>[2x]MKMNVESF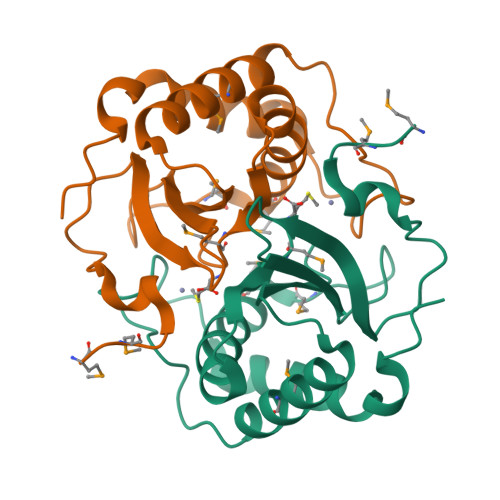NLDHTKVKAPYVRIADRKKGVNGDLIVKYDVRFKQPNRDHMDMPSLHSLEHLVAEIIRNHANYVVDWSPMGCQTGFYLTVLNHDNYTEILEVLEKTMQDVLKAKEVPASNEKQCGWAANHTLEGAQNLARAFLDKRAEWSEVGVGSHHHHHH5-O-phosphono-beta-D-ribofuranose | 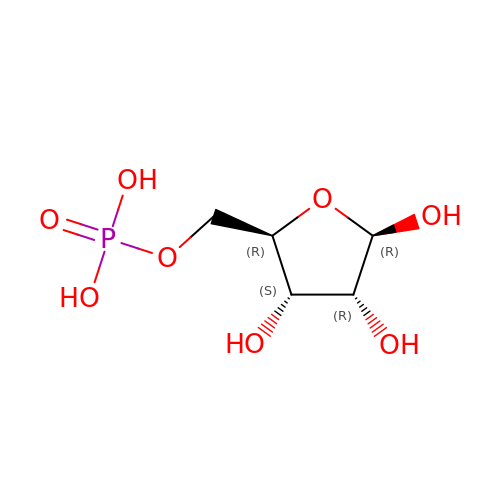C5 H11 O8 P | KTVPXOYAKDPRHY-TXICZTDVSA-N>PEFFSVRHLELAGDDPYSNVNCTKILQGDPEEIQKVKLEILTVQFKKRPRWTPHDYINMTRDCASFIRTRKYIVEPLTKEEVGFPIAYSIVVHHKIEMLDRLLRAIYMPQNFYCIHVDRKAEESFLAAVQGIASCFDNVFVASQLESVVYASWTRVKADLNCMKDLYRMNANWKYLINLCGMDFPIKTNLEIVRKLKCSTGENNLETEKMPPNKEERWKKRYAVVDGKLTNTGIVKAPPPLKTPLFSGSAYFVVTREYVGYVLENENIQKLMEWAQDTYSPDEFLWATIQRIPEVPG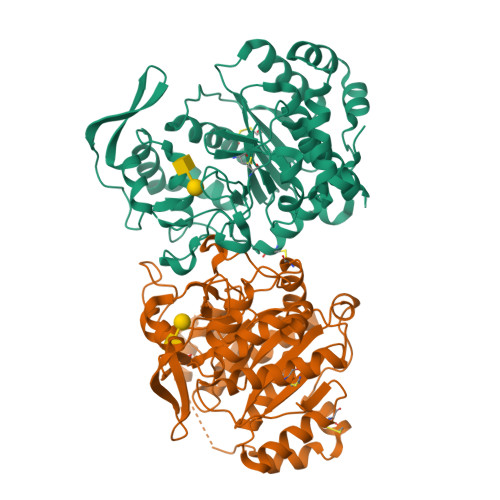SFPSSNKYDLSDMNAIARFVKWQYFEGDVSNGAPYPPCSGVHVRSVCVFGAGDLSWMLRQHHLFANKFDMDVDPFAIQCLDEHLRRKALENLEH[4x]(2S,3S)-3-AMINO-4-(3,3-DIFLUOROPYRROLIDIN-1-YL)-N,N-DIMETHYL-4-OXO-2-(TRANS-4-[1,2,4]TRIAZOLO[1,5-A]PYRIDIN-6-YLCYCLOHEXYL)BUTANAMIDE | C22 H30 F2 N6 O2 | 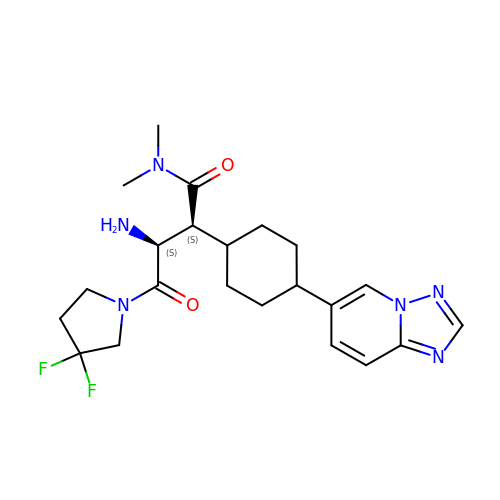JNAZOMVWUGPITI-LNMJFAINSA-N> MLNGASIIVSLFLCFVGGAYACCSEDDCPSGWKFFGGSCYLFDEGSRGWEGSKAFCESKDASLVTVECSKEDDFIRGILSGQTAKHYYWIGARWNEEHNDYRWIDGSPFTFIG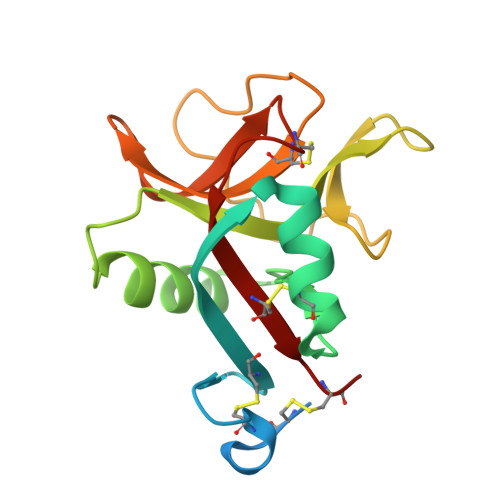WGPGKPDNNKGCLDYLNYKEVVWQWNDHVDCENTNGPCICEIDCSD> HHNGTNGTMMQYFEWHLPNDGNHWNRLRDDAANLKSKGITAVWIPPAWKGTSQNDVGYGAYDLYDLGEFNQKGTVRTKYGTRSQLQGAVTSLKNNGIQVYGDVVMNHKGGADGTEMVNAVEVNRSNRNQEISGEYTIEAWTKFDFPGRGNTHSNFKWRWYHFDGTDWDQSRQLQNKIYKFRGTGKAWDWEVDIENGNYDYLMYADIDMDHPEVINELRNWGVWYTNTLNLDGFRIDAVKHIKYSYTRDWLTHVRNTTGKPMFAVAEFWKNDLAAIENYLNKTSWNHSVFDVPL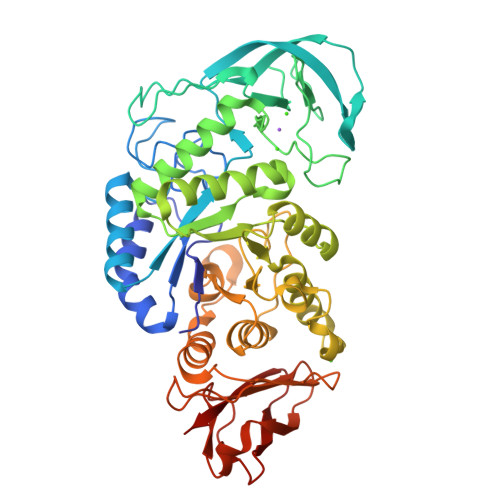HYNLYNASNSGGYFDMRNILNGSVVQKHPIHAVTFVDNHDSQPGEALESFVQSWFKPLAYALILTREQGYPSVFYGDYYGIPTHGVPSMKSKIDPLLQARQTYAYGTQHDYFDHHDIIGWTREGDSSHPNSGLATIMSDGPGGNKWMYVGKHKAGQVWRDITGNRSGTVTINADGWGNFTVNGGAVSVWVKQ>[2x]PASSGLTDETAFSCCSDPDPSTKDFLLQQTMLRIKDPKKSLDFYTRVLGLTLLQKLDFPAMKFSLYFLAYEDK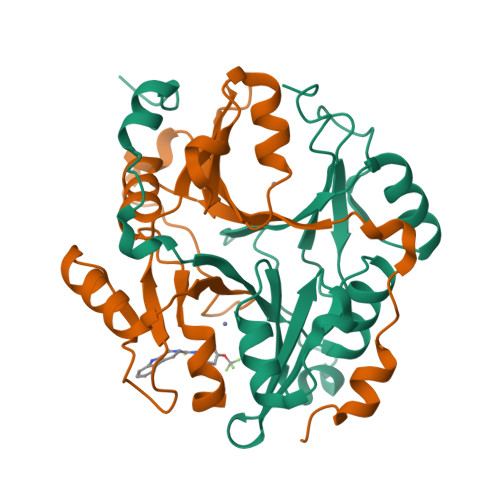NDIPKDKSEKTAWTFSRKATLELTHNWGTEDDETQSYHNGNSDPRGFGHIGIAVPDVYSACKRFEELGVKFVKKPDDGKMKGLAFIQDPDGYWIEILNPNKIATII> EKSVVFKAEGEHFTDQKGNTIVGSGSGGTTKYFRIPAMCTTSKGTIVVFADARHNTASDQSFIDTAAARSTDGGKTWNKKIAIYNDRVNSKLSRVMSPTCIVANIQGRETILVMVGKWNNNDKTWGAYRDKAPDTDWDLVLY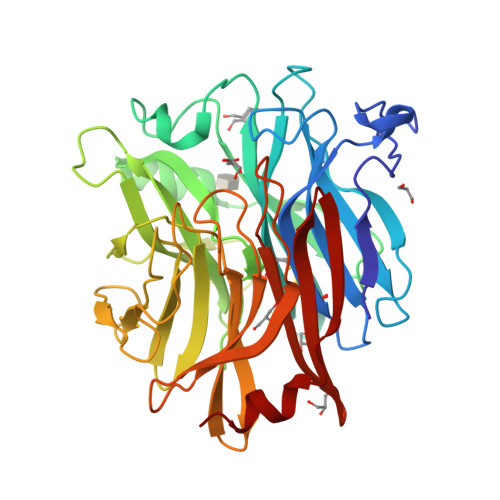KSTDDGVTFSKVETNIHDIVTKNGTISAMLGGVGSGLQLNDGKLVFPVQMVRTKNITTVLNTSFIYSTDGITWSLPSGYCEGFGSENNIIEFNASLVNNIRNSGLRRSFETKDFGKTWTEFPPMDKKVDNRNHGVQGSTITIPSGNKLVAAHSSAQNKNNDYTRSDISLYAHNLYSGEVKLIDDFYPKVGNASGAGYSCLSYRKNVDKETLYVVYEANGSIEFQDLSRHLPVIKSYN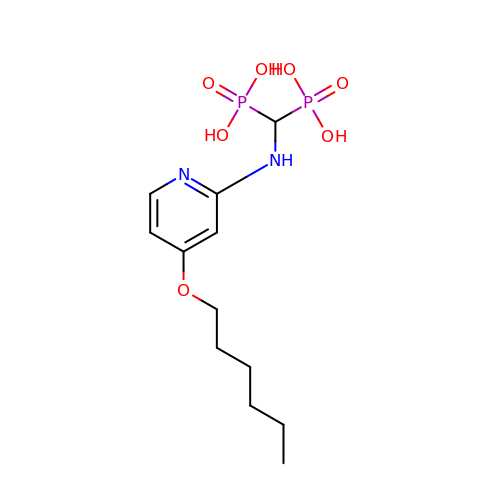[[(4-hexoxypyridin-2-yl)amino]-phosphono-methyl]phosphonic acid | C12 H22 N2 O7 P2 | NXVHNJBPVOSZAP-UHFFFAOYSA-N2-(2-ethoxyethoxy)ethanethiol | C6 H14 O2 S | 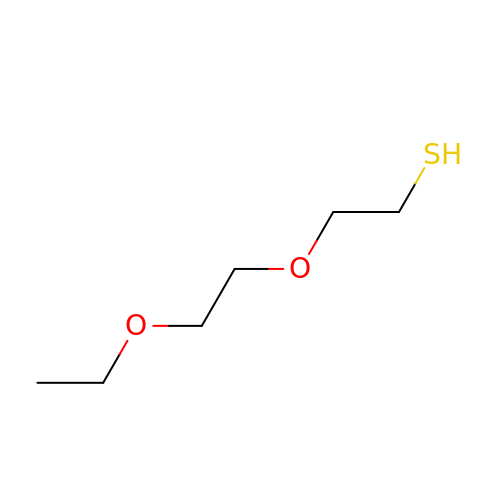LIAMZAFGRCLLJR-UHFFFAOYSA-N> MHHHHHHTLPAFGFAFNASAPQFASLFTPLLLPSVSPNPNIPVPVINDTVSVGDGIRILRAGIYQISYTLTISLDNSPVAPEAGRFFLSLGTPANIIPG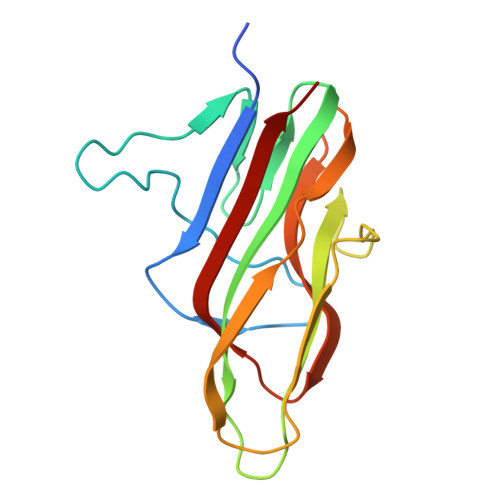SGTAVRSNVIGTGEVDVSSGVILINLNPGDLIQIVPVQLIGTVDIRAAALTVAQIS> LGSPEFLNPQLVQPAKKPYNKIVSHLLVAEPEKIYAMPDPTVPDSDIKALTTLCDLADRELVVIIGWAKHIPGFSTLSLADQMSLLQSAWMEILILGVVYRSLSFEDELVYADDYIMDEDQSKLAGLLDLNNAILQLVKKYKSMKLEKEEFVTLKAIALANSDSMHIEDVEAVQKLQDVLHEALQD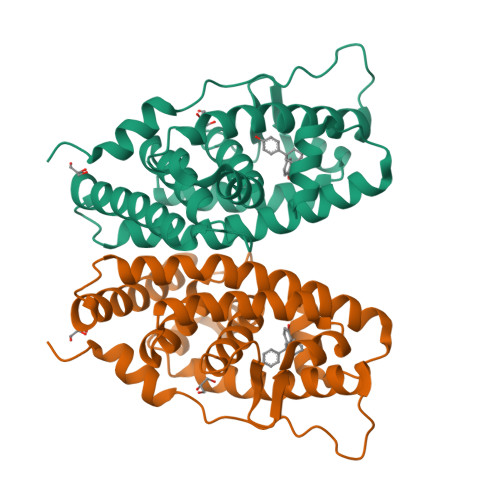YEAGQHMEDPRRAGKMLMTLPLLRQTSTKAVQHFYNIKLEGKVPMHKLFLEMLEAKVC> MNCRSEVLEVSV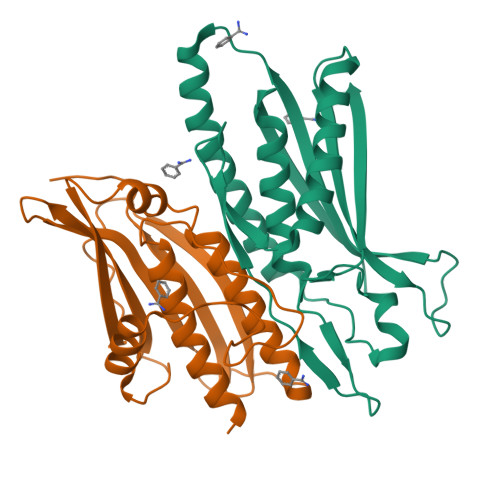EGRQVEEAMLAVLHTVLLHRSTGKFHYKKEGTYSIGTVGTQDVDCDFIDFTYVRVSSEELDRALRKVVGEFKDALRNSGGDGLGQMSLEFYQKKKSRWPFSDECIPWEVWTVKVHVVALATEQERQICREKVGEKLCEKIINIVEVMNRHEYLPKMPTQSEVDNVFDTGLRDVQPYLYKISFQITD;> GAMGSDLDKFIKFFALKTVQVIVQARLGEKICTRSSSSPTGSDWFNLAIKDIPEVTHEAKKALAGQLPAVGRSMCVEISLKTSEGDSMELEIWCLEMNEKCDKEIKVSYTVYNRLSLLLKSLLAITRVTPAYRLSRKQGHEYVILYRIYFGEVQLSGLGEGFQTVRVGTVGTPVGTITLSCAYRINLAFMSTRQ>MKIKNEVMLITYPDSLGSNLKDLKYVLEAHLKEVVGGVHILPFYPSSGDRGFAPMDYTKVDEPFGTWEDIREISNEFYTMYEFMINHISKESVYFKDFIEKKEESPYKDLFIRYSDYWPENRPTERDIDLIYKRKDKAPFIDVTFKDGSTDQVWCTFSEEQIDLDVRTEATRKFVRETLEFLAQQGASIIRLDAFAYAIKKLDTNCFFVEPEIWELLDWCRDILEKHEIVLLPEIHEHYTIQEKIADKGYPVYDFALPMLVLHALYSGRSERLAHWLKACPRKQFTTLDTHDGIGVVDVKDLLTEEEVEFTVNSLYEKGANVKRVYSSEEYNNLDIYQINCTYYSALGNDDQAYLLARAIQMFAPGIPQVYYVGLFAGENDIELLEQTKEGRDINRHYYSLEEIEKELERPVVQELFDLMKFRNQSKAFDGTVDVQTTFDHLLKIT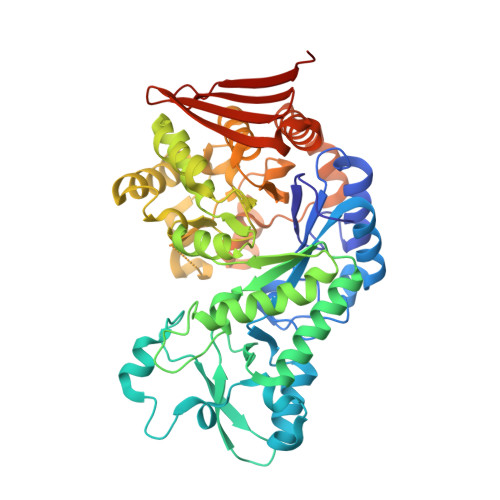WTNGDSKAVLEANLADKTFKIYLEHHHHHH[2x]> ADPPLPEVQCFVFNVEYMNCT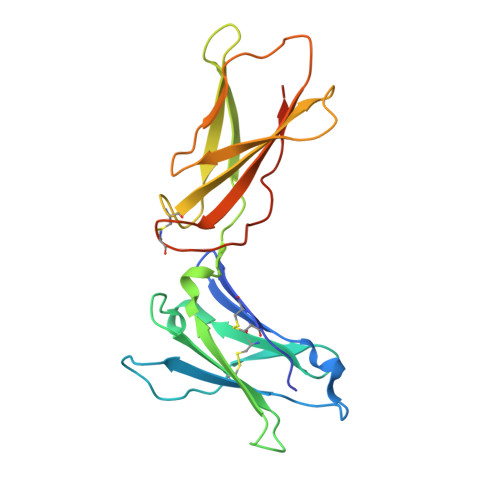WQSSSEPQPTNLTLHYWYKNSDNDKVQKCSHYLFSEEITSGCQLQKKEIHLYQTFVVQLQDPREPRRQATQMLKLQNLVIPWAPENLTLHKLSESQLELNWNNRFLNHCLEHLVQYRTDWDHSWTEQSVDYRHKFSLPSVDGQKRYTFRVRSRFNPLCGSAQHWSEWSHPIHWGSNTSKEN> MGFPASEIKDAVIPEESHLPPIVHVTFMGLYGVTSPLPAHYISDIAQQREGHEAAADFLDIFSHRLITQYYRIWRKYSYPATFEAGGQDKTSQYLLGLARLGIPGCAQNIATPVSRFLALLPLMLLPGRTAEGLTSLVTLLAPGTQARVWHHDRRRIPLKTPLTMRVHHPVSLKSRPVMGDHATDVNGQ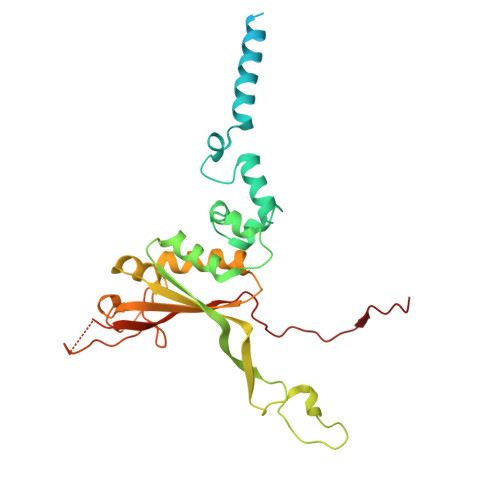VLLQLSTQTGSEVQGWLPGGHLYSDLLALLHVYLGSRLDVRLQLCVERSLLPDARLSCRPAAGSPQLGRTAVMRTQAKIATSAARVMTISLGRYQRVQEHYQRKETQENGDYRW3-ISOPROPYLMALIC ACID | C7 H12 O5 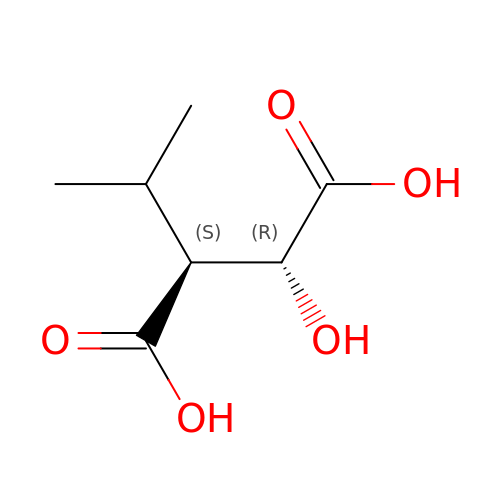| RNQHMTFBUSSBJQ-CRCLSJGQSA-N>[2x]QTPDKAKEQHPKLETYRCTKA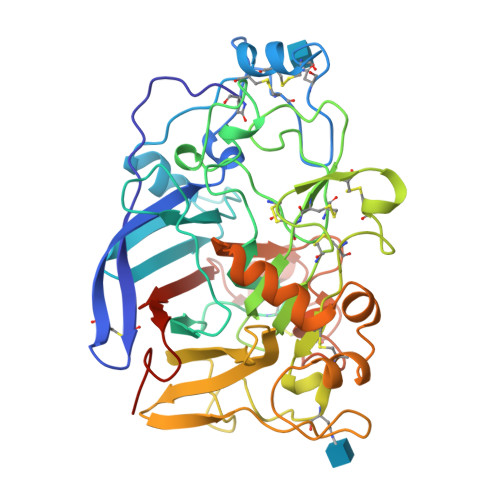SGCKKQTNYIVADAGIHGIRQKNGAGCGDWGQKPNATACPDEASCAKNCILSGMDSNAYKNAGITTSGNKLRLQQLINNQLVSPRVYLLEENKKKYEMLHLTGTEFSFDVEMEKLPCGMNGALYLSEMPQDGGKSTSRNSKAGAYYGAGYCDAQCYVTPFINGVGNIKGQGVCCNELDIWEANSRATHIAPHPCSKPGLYGCTGDECGSSGICDKAGCGWNHNRINVTDFYGRGKQYKVDSTRKFTVTSQFVANKQGDLIELHRHYIQDNKVIESAVVNISGPPKINFINDKYCAATGANEYMRLGGTKQMGDAMSRGMVLAMSVWWSEGDFMAWLDQGVAGPCDATEGDPKNIVKVQPNPEVTFSNIRIGEIGSTSSVKAPAYPGPHRL L-xylulofuranose-1,2-borate 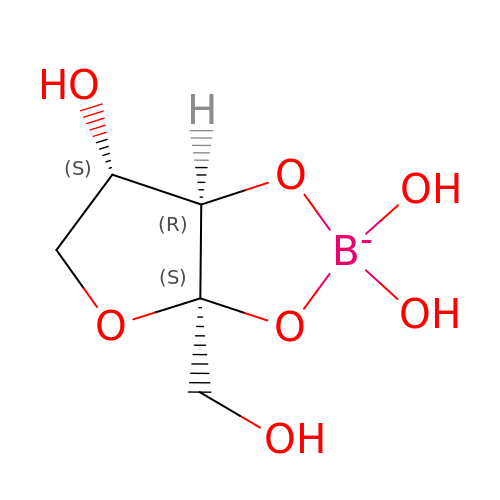| C5 H10 B O7 | HLBKGCVZIOGTKY-VPENINKCSA-N> IHEGPYPEPLVNLLDVVYYGPISIGTPPQDFQVIFDTGSANLWLPSSKCTTKYCLHHHR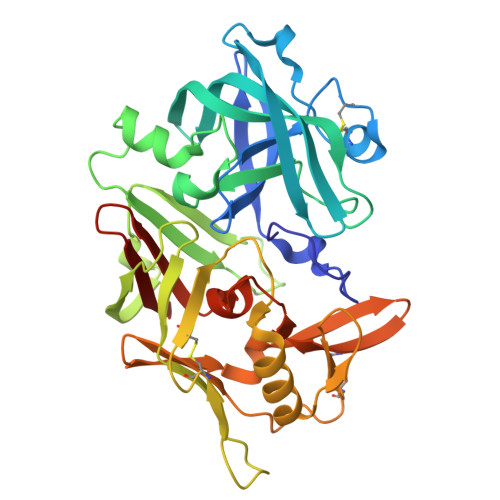YDSSKSSTYEADGRNFTIVYGSGNVEGFISKDVCRIGSAKVSGQPLGEALVVGGESLLEAPFDGILGLAYPSIAVDGVVPVFDNMMKQGLLGEQNVFSVYLNRDPSSKEGGEVLFGGIDHDHYKGSITYVPVTAKGYWQFHVDGVKSVSASKSAPELLCKDGCEAIANTGTSLITGPPEEVDSLNQYLGGTKTEGGQYLLDCDKLESLPNVTFTISGKEFSLRSKDYVLKVNQQGQTLCVSGFMGLEMPQPLWILGDVFLGPYYTIFDRDQDRVGFAEVAHHHHHH I34 formation is essential for viability and catalyzed by adenosine deaminases acting on tRNA (ADATs). In eukaryotes, the essential enzyme catalyzing I34 formation in tRNA is a heterodimer, composed by one active (ADAT2) and one inactive (ADAT3) paralogous subunits, both homologs of the bacterial enzyme. These ADATs carry a characteristic cytidine deaminase (CDA) active-site amino acid signature motif (C/H)XEXnPCXXC (with X being any amino acid, and n being any number of residues), containing the active-site acidic glutamate (inert valine in inactive subunit ADAT3) and cysteine/histidine residues coordinating a Zn2+ cation. To resolve this dilemma, a single tRNA (tRNAArgACG) in bacteria and 7–8 different tRNAs (depending on the organism) with an encoded A34 in eukaryotes (i.e. tRNAThrAGU, tRNAAlaAGC, tRNAProAGG, tRNASerAGA, tRNALeuAAG, tRNAIleAAU, tRNAValAAC, and tRNAArgACG) are post-transcriptionally modified to inosine (I34). This A34 to I34 tRNA deamination leads to the greatest enhancement in decoding capacity that can be caused by a single modification, as the INN anticodon can base pair with three different codon triplets at the mRNA, namely NNC (cytosine-ending), NNU (uracil-ending) and to a lesser extent NNA (adenosine-ending).

Our cryo-electron microscopy (cryo-EM) structure of the tRNA-bound ADAT2/3 from Trypanosoma brucei (T. brucei or Tb) reveals a conserved distortion of the anticodon loop and exposure of the nucleotide bases in common with the bacterial catalytic pocket, with most contacts to the anticodon loop and the target nucleotide A34 provided by the active ADAT2 subunit. The 1:1:1 TbADAT2:TbADAT3:TbtRNAThrCGU complex was reconstituted with in vitro transcribed TbtRNAThrCGU, a non-cognate tRNA omitting the reactive A34 that we chose to stabilize the complex by preventing product turnover. The N-terminal domain of TbADAT3 (TbADAT3N) displayed poorer density, but a DeepEMhancer post-processed map allowed jiggle-fitting the AlphaFold model, without further refinement interventions. The final model comprises the tRNA molecule, TbADAT2 residues 19–103, 123–175, and 183–221, and TbADAT3 residues 1–55, 105–263, and 277–340. In our complex structure, the TbtRNAThrCGU is deeply inserted into the active site of TbADAT2 with all seven nucleotides (32–38) of the anticodon loop interacting directly with the ADAT2/3 deaminase core. Here, the sugar-phosphate backbone adopts a bent conformation and the nucleosides U33, C*34, G35 and A37 are splayed outwards. The nucleobase of U36 is unconventionally internalized via a π-π stacking interaction between the nucleobase of C32 and residue Y205 of ADAT2. Furthermore, the reactive nucleobase C*34 conformation is stabilized through hydrophobic interactions with V46TbADAT2 and V133TbADAT2 as well as hydrogen bonding with the conserved asparagine N79TbADAT2, while its ribose moiety is clamped by V44TbADAT2 and F160TbADAT2.

> MVQDTGKDTNLKGTAEANESVVYCDVFMQAALKEATCALEEGEVPVGCVLVKADSSTAAQAQAGDDLALQKLIVARGRNATNRKGHGLAHAEFVAVEELLRQATAGTSENIGGGGNSGAVSQDLADYVLYVVVEPCIMCAAMLLYNRVRKVYFGCTNPRFGGNGTVLSVHNSYKGCSGEDAALIGYESCGGYRAEEAVVLLQQFYRRENTNAPLGKRKRKD;> GPDSMEEVVVPEEPPKLVSALATYVQQERLCTMFLSIANKLLPLKPHACHLKRIRRSSATRVATAPMDGFAGGVICDKRDSSVATSTISDGCERNSAALGTPAAEKSHVLELLLSVGGPVDSSALKELESAADTTVAVHRVWVPDRAPRSSAEEWTKWCQIWPFATPKPRVPTQLSECEVGSIQRIFRTVVMPLAKRLRTDETLGIAAVLVDPSDGYRVLVSSGEEHALKRGNSAACLGYVSNSGCRKSNRVVLDHPVTFVLKEVTRKQCKDREVEGDASYLANGMDMFVSHEPCVMCSMALVHSRVRRVFYCFPNPVHGGLGSTVSIHAIQELNHHFRVFRCDSRWLSDPEGVSSDHDNPYWEDLTVP>GPQQEDEKMILSFDKAIQYMSKRKIGALITIERHTGLDEYIETGIALDADITGELLINIFIPNTPLHDGAVIVKEGKIAVASAYLPLSESMLIPKEFGTRHRAAVGISEVSDAITIVVSEETGDVSITLDNELMAGLSQQEYLAILRRELI[2x]

The enzyme CdaA, which synthesizes an essential second messenger cyclic di-AMP (c-di-AMP) in many pathogenic bacteria, has emerged as a promising candidate for the development of novel antibiotics. Additionally, c-di-AMP regulates the bacterial stringent response, further underscoring its significance. The synthesis of c-di-AMP is mediated by enzymes possessing a diadenylate-cyclase (DAC) domain.

However, suitable crystallization conditions for unliganded LmCdaA could not be identified. Therefore, structurally related CdaA enzymes from S. pneumoniae, B. subtilis and E. faecium were cloned, overexpressed in E. coli, purified, crystallized and evaluated for diffraction quality. Additionally, we report the first crystal structures of apo CdaA from E. faecium (EfCdaA) and S. pneumoniae (SpCdaA), as well as atomic resolution structures of BsCdaA.>[2x]MQFRSIIRIVGLLLALFSVTMLAPALVALLYRDGAGVPFVTTFFVLLFCGAMCWFPNRRHKHELKSRDGFLIVVLFWTVLGSAGSLPFLIADNPNISVTDAFFESFSALTTTGATVIVGLDELPKAILFYRQFLQWFGGMGIIVLAVAILPVLGIGGMQLYRAEIPGPVKDTKMTPRIAETAKALWYIYLSLTIACAVAFWLAGMTPFDAISHSFSTIAIGGFSTHDASMGYFDSYAINLITVVFLL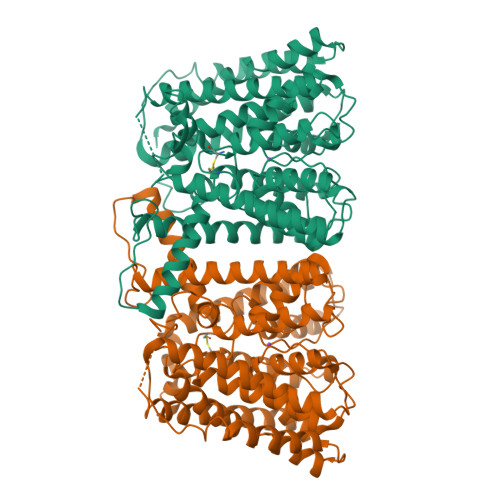ISACNFTLHFAAFASGGVHPKYYWKDPEFRAFIFIQVLLFLVCFLLLLKHHSYTSPYDAFDQALFQTVSISTTAGFTTTGFADWPLFLPVLLLFSSFIGGCAGSTGGGMKVIRILLLTLQGARELKRLVHPRAVYTIKVGGSALPQRVVDAVWGFFSAYALVFVVCMLGLIATGMDELSAFSAVAATLNNLGPGLGEVALHFGDVNDKAKWVLIVSMLFGRLEIFTLLILLTPTFWRSAAAENLYFQ>MKPKEDREWEKFKTKHITSQSVADFNCNRTMNDPAYTPDGQCKPINTFIHSTTGPVKEICRRATGRVNKSSTQQFTLTTCKNPIRCK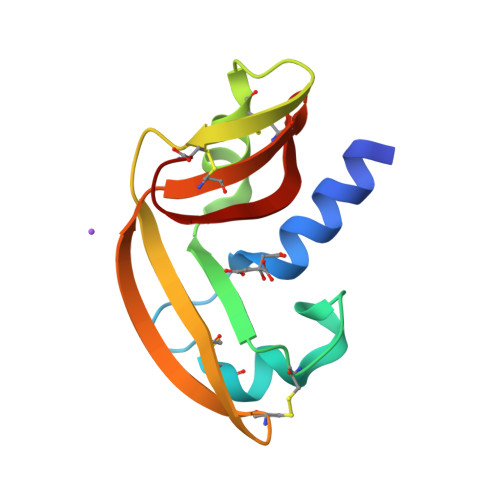YSQSNTTNFICITCRDNYPVHFVKTGKC[2x]>[2x]MSEQSICQARASVMVYDDTSKKWVPIKPGQQGFSRINIYHNTASSTFRVVGVKLQDQQV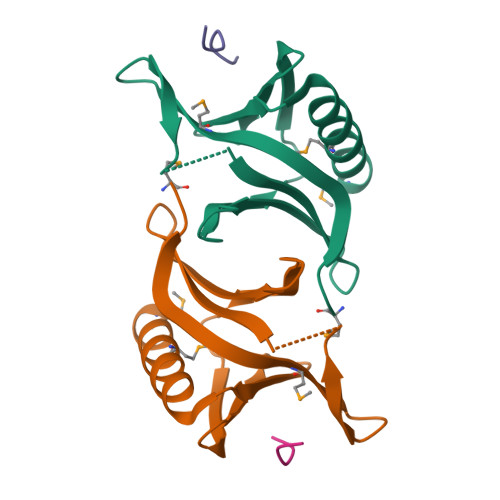VINYSIVKGLKYNQATPTFHQWRDARQVYGLNFASKEEATTFSNAMLFALNIMNSQEGGPSTQRQVQNGPS;>FEFPPPPTDEE[2x]>MQNERSEQSMPGMPAPGLPAGFERRFSRRYAQLDDVRLHYVTGGPDDGEMVVLLHGWPQTWYTWRHVMPALAEDGYRVVAVDYRGAGESDKPLGGYDKASMAGDIRALVHQLGATRIHLVGRSIGVMVAYAYAAQWPTEIVKLAMLDVPVPGTRIWDEAKASADPQIWHFGLHQQRDIAEMLIAGKERAYILDFYKKRTHVALSNDDIAVYADAYAAPGALRAGFELYRAFPQDETRFKAFMKHKLPMPVLALAGDKSNGAKELDMARELALDVRGAVAPNTGHWLPDENPAFLTRQLLDFFREAASGR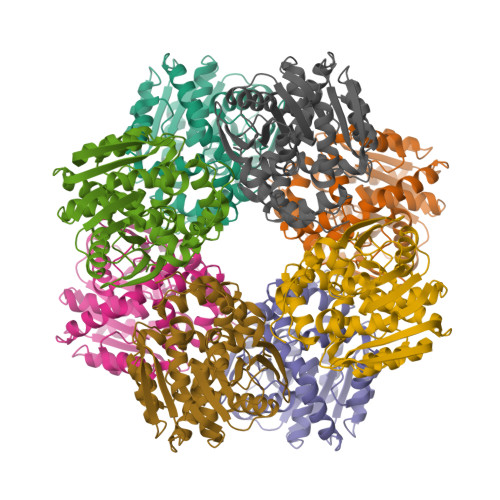[8x]2-methyl-1-(4-{2-[1-(2,2,2-trifluoroethyl)-1H-1,2,4-triazol-5-yl]-4,5-dihydro[1]benzoxepino[5,4-d][1,3]thiazol-8-yl}-1H-pyrazol-1-yl)propan-2-ol 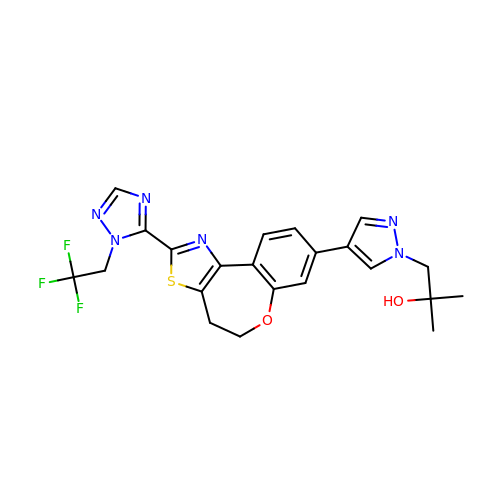| C22 H21 F3 N6 O2 S | VRJUJTMBOARYOG-UHFFFAOYSA-N>MLLFETVREMGHEQVLFCHSKNPEIKAIIAIHDTTLGPAMGATRILPYINEEAALKDALRLSRGMTYKAACANIPAGGGKAVIIANPENKTDDLLRAYGRFVDS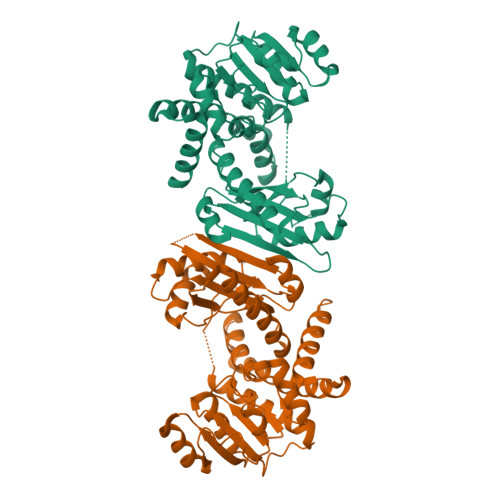LNGRFITGQDVNITPDDVRTISQETKYVVGVSEKSGGPAPITSLGVFLGIKAAVESRWQSKRLDGMKVAVQGLGNVGKNLCRHLHEHDVQLFVSDVDPIKAEEVKRLFGATVVEPTEIYSLDVDIFAPCALGGILNSHTIPFLQASIIAGAANNQLENEQLHSQMLAKKGILYSPDYVINAGGLINVYNEMIGYDEEKAFKQVHNIYDTLLAIFEIAKEQGVTTNDAARRLAEDRINNSKRSKSKAIAALEHHHHHH[6x]> MA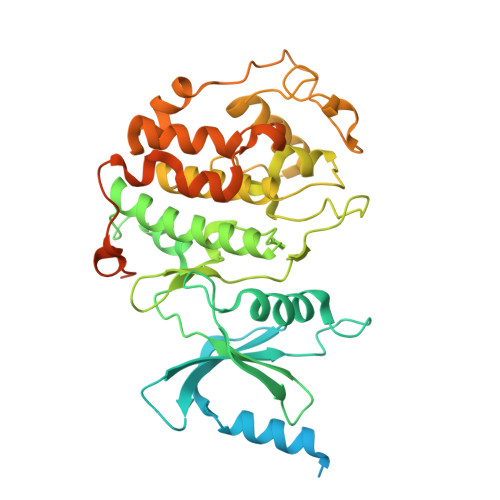ASPLIAPPTDALQQSRPGSTSSPFKRQPQQPSQPPSSTAPSSSNANDTPQLGSRPPNITIANVTSAPFSSRPAITPDPVEQMNEAEKRKYIKGKKLGEGTYANVYLGHSRDDPNFKVAIKKIKVQAQYKDGMAPDAVRELKYLRELRGHPNIIGLISVFSSKDQNLNLVLEYLPLGDLEMLIRDVERVRYGAADIKAWMGMLTRAVWWCHENFILHRDIKPNNLLIAADGEVKLADFGLARSFADPGRRMTANVITRWYRPPELLFGARHYGGAVDIWSVGMVFAELIIRSPFLPGNTEMEQITLICKHIGTPTEENWPGVSKLPEWWDPMEEPIPVWGKDAYMARFGAVGSEGVDLLWRTLQLDPKKRITAREMLEHRWWRTDPKPTRKEDLPKKSGGEDKMGADLKRRPGMVEDENGPRGSKVARKLDFGQLK>VQAANLMDRIKANPVSEKNIDEKFIYNTADFSIELFKNSIDDKENSLISPLSAMLALAMTANGADNETLAQMEKALGKDISIEDLNKYLYTYMKKLPNEEKSKLTIANSIWFKENDFMPSKDFLQIIADYYKADIFKAAFDSSTVSDINNWVKSKTNGMIDKILNKIDPEDVMYLINAVAFDAEWETVYEKASVHEDIFTDVYGNRQKVEFMNSEENLYIEEENAIGFVKPYAKNHYSFVAILPDENISVNEYIKTLTGQKFID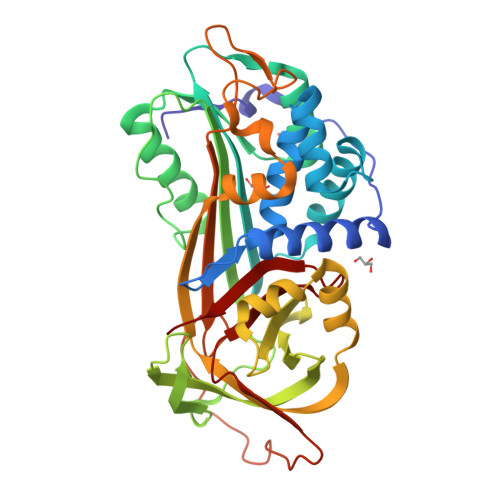LIKNAKITLVRASLPKFKYEYTIKMNETLESLGMTDAFLPDKADFSKLGKSDIGNLYISEVLHKTFISVDELGTKAGAVTSVDITAAGIPVNFKTVKLNRPFIFAIIDNSTNLPIFIGTVLSL[2x]> MGPYRRLWFTLIAVLAVTFALLGFYGGEVYRQAPPIPEEVASADGTRLFGRDDILDGQTAWQSIGGMQLGSIWGHGAYQAPDWTADWLHRELMAWLDLAARDAHGRDYGQLDAPAQAALREQLKAEYRANRADAAGGKLTLSPRRAQAVAQTEAYYDQLFSDAPALHRSRENYAMKENTLPDANRRRQMTHFFFWTAWAAGTEREGTSVTYTNNWPHEPLIGNHPSSENVMWSIISVVVLLAGIGLLIWAWAFLRGKEEDEPPAPARDPLTTFALTPSQRALGKYLFLVVALFGFQVLLGGFTAHYTVEGQKFYGIDLSQWFPYSLVRTWHIQSALFWIATGFLAAGLFLAPLINGGRDPKYQKAGVDILFWALVLVVVGSFAGNYLAIAQIMPPDLNFWLGHQGYEYVDLGRLWQIGKFAGICFWLVLMLRGIVPALRTPGGDKNLLALLTASVGAIGLFYGAGFFYGERTHLTVMEYWRWWIVHLWVEGFFAVFATTALAFIFSTLGLVSRRMATTASLASASLFMLGGIPGTFHHLYFAGTTTPVMAVGASFSALEVVPLIVLGHEAWENWRLKTRAPWMENLKWPLMCFVAVAFWNMLGAGVFGFMINPPVSLYYIQGLNTTPVHAHAALFGVYGFLALGFTLLVLRYIRPQYALSPGLMKLAFWGLNLGLALMIFTSLLPIGLIQFHASVSEGMWYARSEAFMQQDILKTLRWGRTFGDVVFLLGALAMVVQVILGLLSGKPAAAEPVLRAEPARRL

A quinol-dependent nitric oxide reductase (qNOR) plays a critical role in the survival of the bacterium in the human host by combatting the host’s immune response. qNORs belong to the broader family of nitric oxide reductases (NORs). NORs are largely found as the essential component of anaerobic nitrate respiration, also known as denitrification, in the bacterial cytoplasmic membrane and catalyse the reduction of nitric oxide (NO) to nitrous oxide (N2O). Whilst cNORs are pre­dominantly found in denitrifying organisms as a respiratory enzyme, qNORs are also found in several pathogenic bacteria, including the Gram-negative, human-pathogenic bacterium N. meningitidis, as an enzyme that is responsible for the detoxification of NO produced by the host. High-resolution structure determination of N. meningitidis qNOR (NmqNOR) is of importance to provide a framework for developing a knowledge-based strategy for the design of new antibacterial agents, as well as to help to understand the chemistry of NO reduction, 2NO + 2 H+ + 2e− → N2O + H2O, at the heme and nonheme iron (FeB) binuclear centre.

We chose the Glu494Ala mutant of AxqNOR, which primarily migrated as a monomer on a chromatographic column, to define a cryo-EM structure of a monomeric qNOR. TMIX, which contains two of the three FeB ligands, His537 and His538, is very distorted. Regardless, they cause more pronounced changes of the dimer-stabilization and proton channel-flanking helices, confirming Glu494 to be a critical residue not only for activity but also for structural maintenance of the dimer and active site in AxqNOR. The single mutation results in active-site disturbance of nonheme iron ligands, culminating in displacement of the dimer-stabilizing TMII and the putative proton-transfer channel flanking helices TMIX and TMX, acting to create a catalytically inert monomeric qNOR.>[2x]ADTQGYKWKQLLYNNVTPGSYNPDNMISTAFAYDAEGEKLFLAVPRKLPRVPYTLAEVDTKNSLGVKGKHS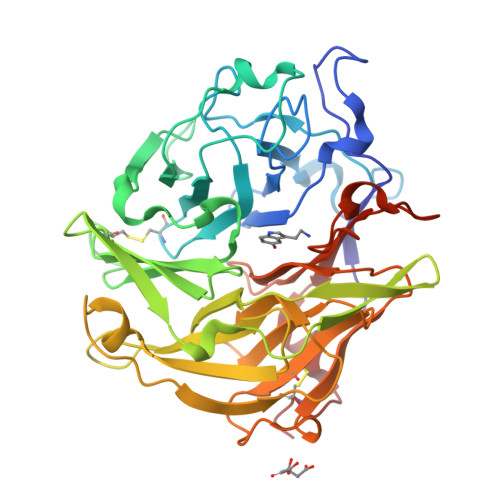PLLNKFSGHKTGKELTSIYQPVIDDCRRLWVVDIGSVEYRSRGAKDYPSHRPAIVAYDLKQPNYPEVVRYYFPTRLVEKPTYFGGFAVDVANPKGDCSETFVYITNFLRGALFIYDHKKQDSWNVTHPTFKAERPTKFDYGGKEYEFKAGIFGITLGDRDSEGNRPAYYLAGSAIKVYSVNTKELKQKGGKLNPELLGNRGKYNDAIALAYDPKTKVIFFAEANTKQVSCWNTQKMPLRMKNTDVVYTSSRFVFGTDISVDSKGGLWFMSNGFPPIRKSEKFKYDFPRYRLMRIMDTQEAIAGTACDMNA> DFQSESYKDAYSRINAIVIEGEQEAFDNYNRLAEMLPDQRDELHKLAKMEQRHMKGFMACGKNLSVTPDMGFAQKYYERLHENFKAAAAEGKVVTCLLIQSLIIECFAIAAYNIYIPVADAFARKITEGVVRDEYLHRNFGEEWLKANFDASKAELEEANRQNLPLVWLMLNEVADDARELGMERESLVEDFMIAYGEALENIGFTTREIMRMSAYGLAA;> LDFQS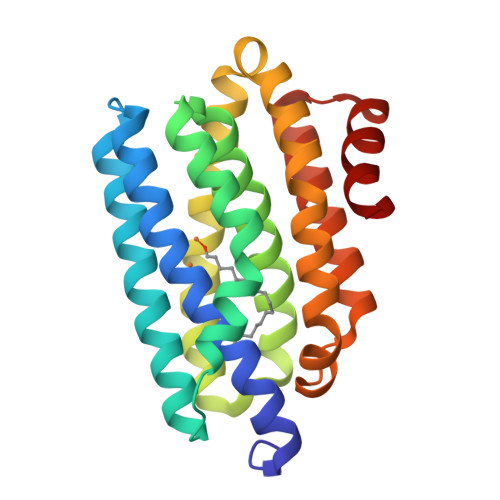ESYKDAYSRINAIVIEGEQEAFDNYNRLAEMLPDQRDELHKLAKMEQRHMKGFMACGKNLSVTPDMGFAQKYYERLHENFKAAAAEGKVVTCLLIQSLIIECFAIAAYNIYIPVADAFARKITEGVVRDEYLHRNFGEEWLKANFDASKAELEEANRQNLPLVWLMLNEVADDARELGMERESLVEDFMIAYGEALENIGFTTREIMRMSAYGLAAV Bile salt hydrolases (BSHs) comprise a diverse family of microbial enzymes that catalyse critical BA transformation. Primary conjugated BAs synthesized in the liver, such as the tauro- and glycoconjugates of cholic acid (TCA, GCA), are deconjugated by BSHs to generate cholic acid (CA) (BA names and abbreviations are summarized in Supplementary Fig. 1). We found that Lactobacillaceae BSHs display a clear bias for either glycine or taurine-conjugated BAs. Notably, each monomer contains a loop that swaps into the active site of a neighbouring monomer within the tetramer and places amino acids proximal to the catalytic residues.

To examine the molecular foundations of BSH substrate specificity, we determined the crystal structures of six of the Lactobacillaceae BSHs examined above: four glycine-preferring (LgasBSHb, LaciBSHa, LingBSH, LreuBSH) and two taurine-preferring (LgasBSHa, LjohBSHc) BSHs. We examined the sequences of these loops and found that taurine-preferring enzymes exclusively contained G-V/T-G (‘G-X-G’) motifs, while glycine-preferring enzymes solely contained S-R-G/S (‘S-R-X’) motifs. To confirm the importance of the selectivity loop, we first created two variant enzymes that swap the central residues in each selectivity loop: a V211R mutant of the taurine-preferring LgasBSHa and a R208V mutant of the glycine-preferring LgasBSHb. We found that both single-swap mutations significantly decreased the specific activities with preferred substrates without significantly impacting the non-preferred substrate. Second, we noted that R208 in LgasBSHb forms a salt bridge with E21, an anionic residue conserved in all glycine-preferring enzymes examined; in taurine-preferring BSHs, this glutamate is always replaced by glycine. We examined the activity of LgasBSHa G23E and LgasBSHb E21G variants and found that they decreased activity with the preferred substrate without impacting non-preferred substrate activity. Third, combining these mutations by adding a G23E V211R salt bridge in LgasBSHa further lowered the preferred activity, while removing the salt bridge in LgasBSHb E21G R208V did not further decrease the preferred activity. Fourth, we created triple mutants of the selectivity loop sequence. Both the LgasBSHa-SRS and LgasBSHb-GVG variants exhibited the greatest reduction in specific activities toward their preferred substrates, with little effect on non-preferred substrate processing. Importantly, without altering secondary structure, the triple mutations significantly decreased substrate selectivity from 76-fold to 14-fold for LgasBSHa and from 353-fold to 2-fold for LgasBSHb.

>MCTSILYSPKDHYFGRNLDYEIAYGQKVVITPRNYEFKFANLPAEKSHYAMIGIAAVANNTPLYCDAINEKGLGVAGLSFAGQGKYFPVVEDKKNIASFEFISYILATYETVDQVKENLTDVNISDVSFSKNTPASELHWLVGDKTGKSIVVESDEKGLHVYDNPVNALTNAPLFPQQLTNLANYAAVVPGQPNNDFLPGVDLKMYSRSLGTHHLPGGMDSESRFVKVCFALNHAPKDSDEVESVTNFFHILQSVEQVKGMDEVGPNIFEYTMYTSCMNLEKGILYFNCYDDSRISAVDMNKEDLSSSDLIVFDLFKKQDISFINHHHHHH[8x]(1R,4'S)-3,4-dihydro-2H-spiro[naphthalene-1,3'-pyrrolidin]-4'-yl[(2S,4R)-2,4-diphenylpiperidin-1-yl]methanone 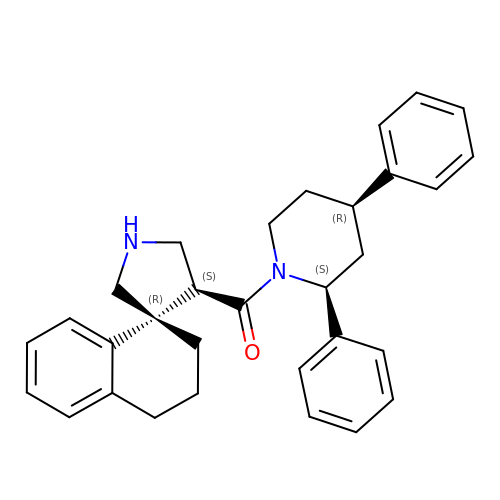| C31 H34 N2 O | MXPUWFOJTXJTTA-RNWXARPHSA-N Glutamine synthetases (GS) catalyze the ATP-dependent ammonium assimilation, the initial step of nitrogen acquisition that must be under tight control to fit cellular needs. The dodecamer is organized as two stacked hexameric rings, and each polypeptide is organized into two parts, a shorter N-terminal domain (β-Grasp fold) and the remaining C-terminal domain. The active sites are located at the interface of the N- and C- terminal domains of the adjacent subunit in the hexameric ring. Two loops in the active center are critical for catalysis: the Glu-flap, involved in shielding the active site during catalysis and deprotonating the intermediate product, and the Asp-50’ loop, which binds and deprotonates ammonium.

The enzyme from M. shengliensis was crystallized in the absence of ligands, and two different crystalline forms, referred to as MsGS-apo 1 and MsGS-apo 2, were analyzed. MtGS-apo-TbXo4 was selected as a template for molecular replacement, and the structures were refined to 2.64 Å and 3.09 Å, respectively. As MtGS, the homolog from M. shengliensis has a dodecameric organization with the N-ter (1-106) and C-ter (107-442) domains forming the protomeric unit. MsGS-apo 1 was used for the following structural analyses due to the better resolution. A structural comparison of the monomeric unit reveals that MsGS has a closer fit with BsGS compared to MtGS (rmsd MsGS-BsGS: 0.749 Å, 341 atoms aligned, MtGS-BsGS: 0.847 Å, 338 atoms aligned), which exhibits larger deviations such as an extended helix α2 resulting from a seven-residue insertion. Unlike for MtGS, 2OG was not required for MsGS activity, and its addition (2 mM) did not affect its activity. In the 2OG-insensitive MsGS structure, the side chain of Glu89ʹ substituting the MtGS Val94ʹ would collide with the 2OG position, and its negative charge would additionally lead to the ionic repulsion of 2OG. Moreover, in MsGS, most of the residues relevant for 2OG coordination (Arg88ʹ, Arg174 and Ser191) are substituted. The Arg62ʹ is not conserved in MtGS (substituted by Gly67ʹ) but is present in MsGS (Arg61ʹ). As suspected from the sequences, the addition of glutamine (20 mM) inhibited the activity of MsGS by 97%, while no difference was observed for MtGS.

>[12x]MGSKEDEIFRIVEEKNVRFVRLQFVDVQGIPKNVAIPVGQLEKALGPGIHFDGSSIEGFVRIEESDMVLRPDPDTFRVLPWSGNEGTAEARLICDIELPDGKPFMGCPRQVLKKNMEEAAKLGYVMNTGPEMEFFLFKRQDGMPTNIPQDRGGYFDLAPIDLAEEIKREIVLVLEEMGFEVEAAHHEVAFGQHEIDFKYDNALATADNVITLKYVAKTLALQHGLHATFMPKPIFGVNGSGMHTNTSLFKDGKNAFYDPDAPDQISDTLRYFVGGVLKHIRAITAITNPLVNSYKRLVPGYEAPVYITWSGPNRSSLIRVPAPRGNSTRIEIRSPDPSCNPYLAFAAILAAGLDGVKNKIEPPERVEKNIYKLTEEEREKLGIGMLPGTLKEAIECFKEDELLVSALGEHVSQSIINVAMADWDSYRTQVHQWELDRYLQTY>[2x]MM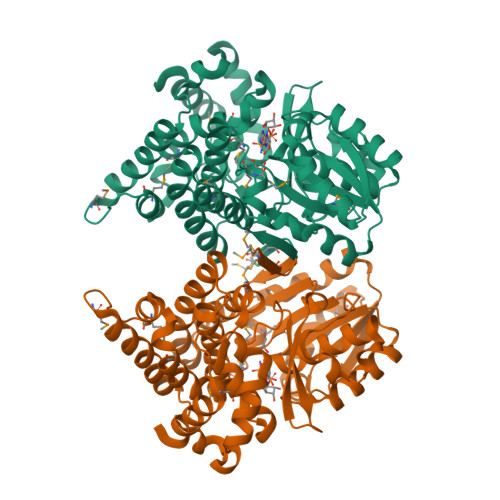ANRMILNETAWFGRGAVGALTDEVKRRGYQKALIVTDKTLVQCGVVAKVTDKMDAAGLAWAIYDGVVPNPTITVVKEGLGVFQNSGADYLIAIGGGSPQDTCKAIGIISNNPEFADVRSLEGLSPTNKPSVPILAIPTTAGTAAEVTINYVITDEEKRRKFVCVDPHDIPQVAFIDADMMDGMPPALKAATGVDALTHAIEGYITRGAWALTDALHIKAIEIIAGALRGSVAGDKDAGEEMALGQYVAGMGFSNVGLGLVHGMAHPLGAFYNTPHGVANAILLPHVMRYNADFTGEKYRDIARVMGVKVEGMSLEEARNAAVEAVFALNRDVGIPPHLRDVGVRKEDIPALAQAALDDVCTGGNPREATLEDIVELYHTAWEGG>[3x]GLKGQEFAPSHQQVYAPLRADGDKPRAHLTVVRQTPTQHFKNQFPALHWEHELGLAFTKNR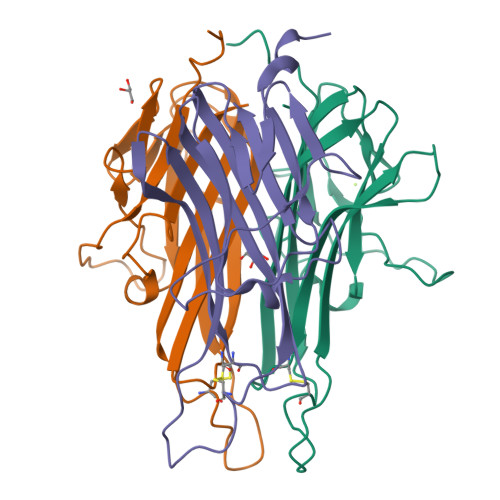MNYTNKFLLIPESGDYFIYSQVTFRGMTSECSEIRQAGRPNKPDSITVVITKVTDSYPEPTQLLMGTKSVCEVGSNWFQPIYLGAMFSLQEGDKLMVNVSDISLVDYTKEDKTFFGAFLL> GAMSVASLPECVKNFFPTEQLEFSSSITADEKPVLHEVFQKHSCFSQCGEMIDEVSKKHPELGKRLATVLEGNK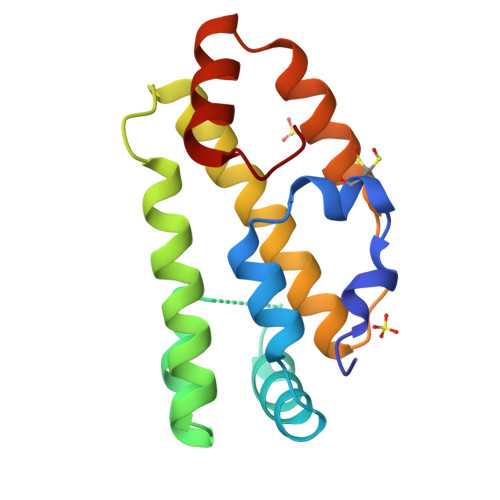KRLDGLSPAAVEYAKKLIHMVTTTLCSLTVGKPIDDADAKRLHQEFQSLSSEDQAALRKNNPDIKF> MGSSHHHHHHSQDPMQHIIPLTITFLESFRVIEWHKSSDRNSLRFLRGYAYARWHRSLKNNKGRPYITGTLVRSAIIRAAEELLWLNDGNYKGAICCPGEFNGSNAKVFREGKARRLRRRQTLTWPTKCACHEKEPCPFCLLLGRYEKSSKTSKSPVLNNVNFSNFNVLGKEKEFLNIEDVADMRVVNRVDQQSGKAEDFFNIWEITDGAWKIFRGEIQVSDKGWSDEENFSKFLTLLKGASVLVDKISGGLCYLTLDKPELAELPAVKTEKDVLEPGDDASVLEISRPPYWNNMLNLAGTISEAFEREDKLVHLRLFADTVRELRRSDIETLDLPKGHADRLGKPSDHFIWDIEINKKVKLRNWLFWIFNEFRDTYAYFDWRTFCEALGQALYLEAKKQVPNQFSSERPVGATPAMEVKTPEHDPGRAAQGPRYEWLIKGELVSQTPFFFGWSTEADNREHTNLKLLAARDGRLRLPLSVLRGILRRDIKVVLDNKCRAELAMKQPCSCPVCNLMKKITIRDSFSSNYAEPPKIRHKIRLDPKSGTVAKGALFDSEVGPRGVVFPFELRLRSADDTLPQALKTVFSWWQQGTVSFSGDAGTGKGIFCLRNLKSIRWDLKTEMDKYAATLGGRKTPV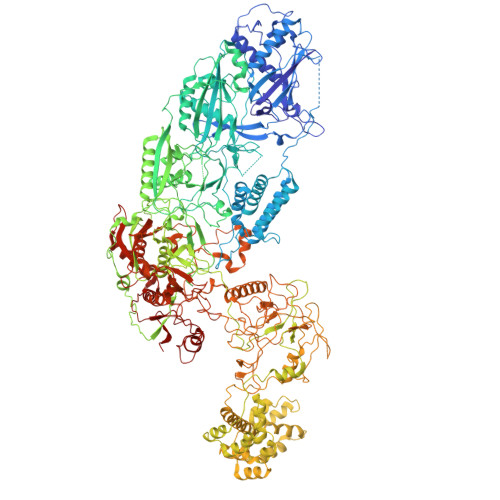GKWDKCHIPDDKTYPWVKETVEISVCSPFITKDPVNSLIDSAGYDAICYTTVDLEKSENINSLPESEISLLFEMFDLQYPMSYLFPNKDIYLLKGESFRGMLRTAVGRGENLLLREHEDCSCTLCRIFGNEHNAGKIRVEDFIIQGEPRTKLVDRVAIDRFTAGAKDKFKFDAAPIVGTPTNKLKFRGNIWIHRDLDGLACESLKLALEDIENGLYPFGGLGNAGFGWVNYNPLSHPAQEENKADFSLTKKMELNWSMKELSTDKIYWPHYFLPFGKKVLREKTPPSHACIDENEDSELYSGKIVCTLETRTPLIIPDSEFQGEEHKSYDFFNLNGELCIPGSEIRGMISSVFEALTNSCMRIFDEKKRLSWRMNPNKKDKKNNNRRELDDFIPGRVTNDRKMEEMKEYRYPFYDQAITANDKQNKYFDQWEATIELTDESLEKLKAEKILQSVLDALRPLTKKKEKYKNTETFVFDLKKFIGKIDDNQQMISEALERGKVRLTGNSLKQISKTKKIPRQILNQLKGLKDNTYENREQFISVLKTTVRGINDEQISLILDNIDEDVRLTDLSLTKIRKAKVPQTLVDMLADLKKDEPYKNEKEFLSEFKKKMGEIIGLILKHAAKTGGDVPRYNHPTPTDKMLLSLAAYNRNHKHENGKAEYRIVKPKHNLKVDFMFAVTPFENPFKGYNPAAVVEEPVGGYLKVSGPNKIEKVKKVNPNSVSVRDDKNQEIIHNGVYLRKITVANAKSKNKLRERLVPEFAWYDKDSEAAYAMTKRCERVFVEIGAKPIPIQPSAREKFKILTQEYQKNAKQQKTPEAFQTILPKDGELRPGDLVYFREDKKTNTVTDIIPVRISRTVDDEVLARKIPDDVGDVRPCVREILDKEKQKEIADAGVKEVFQHHPDGLCPACSLFGTTFYKGRIAFGFAFHKDKDPELANNGKHITLPLLERPRPTWSMPKKESRVPGRKFYVHHQGWERVIKHSNLDESDPNATKQTVNNRSVQAIKEEQKFQFEVRFENLREWELGLLVYVLQLEPQFAHKLGMGKALGFGSVRIRVGEIHSGPKELDESRLVSSAMKKMEEIWDRDKNVLEKLFRLLYFNESKDIKVRYPKLQKEKEEEEEESGYMELAKEEYQPEQRRNKLTNPWEGWGNILKKPAILI> MSLDFRSADFLRTHISDTMAFYHPRCIDSAGGFFHYFRDDGSIYNATHRHLVSSTRFVFNYAMAYLQFGTAEYLDAVHHGLSYVRDVHRNPATGGYAWTLCDDRVEDDTNHCYGLAFVMLAYSCGLKVGIKQAREWMDETWCLLERHFWDAEYGLYKDEADAQWNFTRYRGQNANMHMCEAMLAAYEASGEQRYLERALVLADRITRRQAAKADGLVWEHYDMRWEVDWDYNRDNPKHLFRPWGFQPGHQTEWAKLLLILDRYIEVE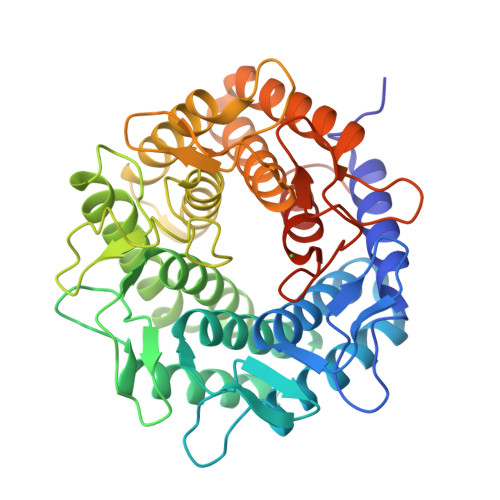WLVPVARSLFDVAVARSWDAVRGGLCYGFAPDGTICDDDKYFWVQAESLAAAALLATRSGDERYWQWYDRLWAYAWQHMVDHRYGAWYRLLDGDNRKYNDEKSPAGKTDYHTMGACHEVLNVVWTKSEGHHHHHH methyl [(2S)-2-(5-{5-[4-({(2S)-2-[(3S)-3-amino-2-oxopiperidin-1-yl]-2-cyclohexylacetyl}amino)phenyl]pentyl}-2-fluorophenyl)-3-(quinolin-3-yl)propyl]carbamate 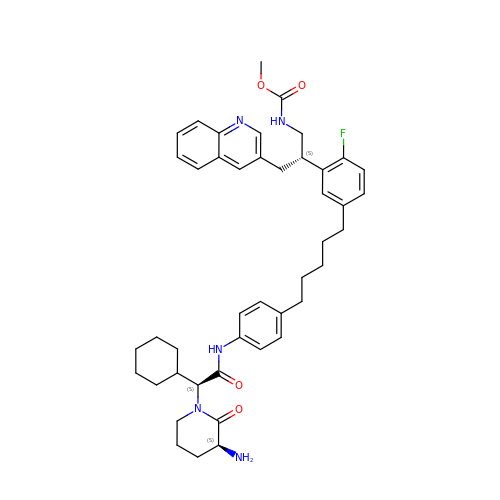| C44 H54 F N5 O4 | SDVPSGCYRLUZSS-WXSHXSFMSA-N> SNAMNQQPIKIAVFGLGGVGGYYGAMLALRAAATDGLLEVSWIARGAHLEAIRAAGGLRVVTPSRDFLARPTCVTDNPAEVGTVDYILFCTKDYDMERGVAEIRPMIGQNTKILPLLNGADIAERMRTYLPDTVVWKGCVYISARKSAPGLITLEADRELFYFGSGLPEQTDDEVRLAELLTAAGIRAYNPTDIDWYIMKKFMMISVTATATAYFDKPIGSILTEHEPE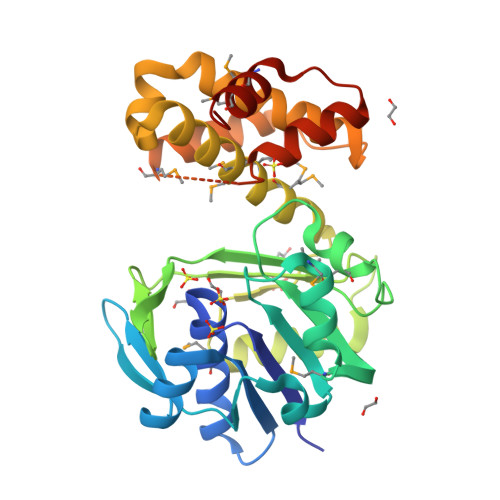LLSLLEEVAELFRAKYGQVPDDVVQQLLDKQRKMPPESTSSMHSDFLQGGSTEVETLTGYVVREAEALRVDLPMYKRMYRELVSRTAN> MVCKVCGQKAQVEMRSRGLALCREHYLDWFVKETERAIRRHRMLLPGERVLVAVSGGKDSLALWDVLSRLGYQAVGLHIELGIGEYSKRSLEVTQAFARERGLELLVVDLKEAYGFGVPELARLSGRVACSACGLSKRYIINQVAVEEGFRVVATGHNLDDEAAVLFGNLLNPQEETLSRQGPVLPEKPGLAARVKPFYRFSEREVLSYTLLRGIRYLHEECPNAKG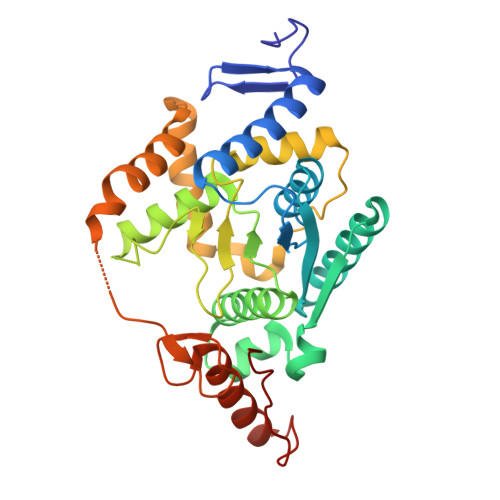AKSLLYKEALNLVERSMPGAKLRFLDGFLEKIRPRLDVGEEVALRECERCGYPTTGAVCAFCRMWDAVYRRAKKRKLLPEEVSFRPRVKPLRAG> MASNAARVVATAKDFDKVGLGIIGYYLQLYAVELILSEEDRSQEMTALATELLDTIEAFKKEIGGESEAEDSDKSLHVMNTLIHDQEKAKIYMLNFTMSLYNEKLKQLKDGPWDVM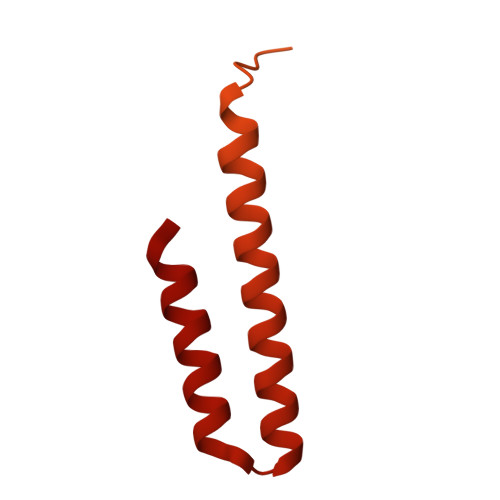LKRSLWCCIDLFSCILHLWKENISETSTNSLQKRIKYCKIYLSKLAKGEIGSSDEKTLDYADFADDSEEIKDEDVDHQTSDLENNNNDKVEGLAPKDQTTSYEPVDEVPEFIDDADSVNEEEQTVDKNEDAITKDEQQVVKKEVDLTRPSAPSEPAAAEHKSYTKDELTKIMDRASKIEQIQKLAKYAISALNYEDLPTAKDELTKALDLLNSI>[2x]MTKAKDLTGKKIAILAADGVEEIELTSPRAAIEAAGGTTELISLEPGEIQSMKGDIEPQEKYRV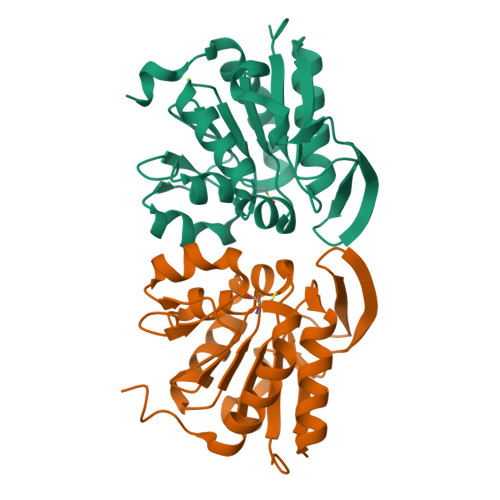DHVVSEVQVSDYDGLLLPGGTVNPDKLRLEEGAMKFVRDMYDAGKPIAAICHGPWSLSETGIAQGLKMTSWSSLKRELTLAGAQWVDEECVTDKGVVTSRKPDDLPAFNKKIVEEFAEGDHSSRRK> MQKLTVGLIGNPNSGKTTLFNQLTGARQRVGNWAGVTVERKEGIFATTDHQVTLVDLPGTYSLTTISSQTSLDEQIACHYILSGDADML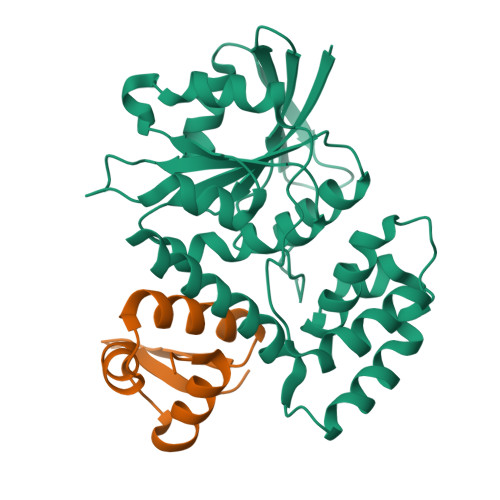INVVDASNLERNLYLTLQLLELGIPCVVALNMLDIAEKQQVRIDIDALAARLGCPVIPLVSTRGRGIEALKIALDRHQANSDLELVHYPQPLLREADLLAQQMSAQIPPRQRRWLGLQMLEGDIYSRAYAGDAADKLDIALANLSDEIDDPALHIADARYQTIAAICDAVSNTLTAEP;> GPLGSMASLMEVRDMLALQGRMEAKQLSARLQTPQPLIDAMLERMEAMGKVVRISETSEGCLSGSCKSCPEGKAACRQEWWALRL> MRVLVTGGSGYIGSHTCVQLLQNGHDVIILDNLCNSKRSVLPVIERLGGKHPTFVEGDIRNEALMTEILHDHAIDTVIHFAGLKAVGESVQKPLEYYDNNVNGTLRLISAMRAANVKNFIFSSAATVYGDQPK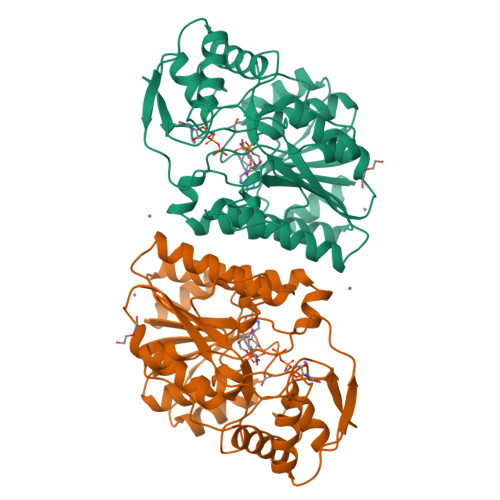IPYVESFPTGTPQSPYGKSKLMVEQILTDLQKAQPDWSIALLRYFNPVGAHPSGDMGEDPQGIPNNLMPYIAQVAVGRRDSLAIFGNDYPTEDGTGVRDYIHVMDLADGHVVAMEKLANKPGVHIYNLGAGVGNSVLDVVNAFSKACGKPVNYHFAPRREGDLPAYWADASKADRELNWRVTRTLDEMAQDTWHWQSRHPQGYPD>[41x]TTTATDLMKSGDATVKGTFG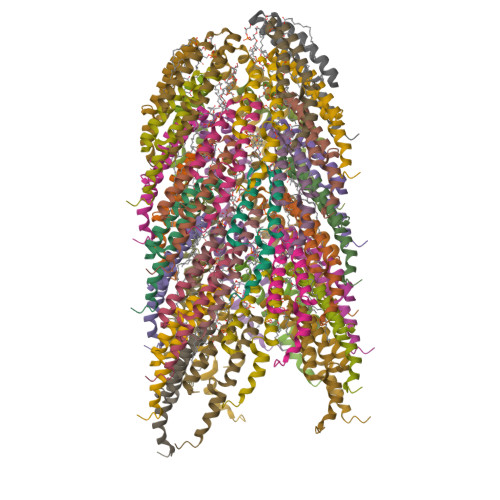KQSSVVKWVVLAEVVAGGIMYMMTKNVKFLFGFAIISTFITIGMSVAGY>[20x]MSEKRVQPLARDAMAYVLAGGRG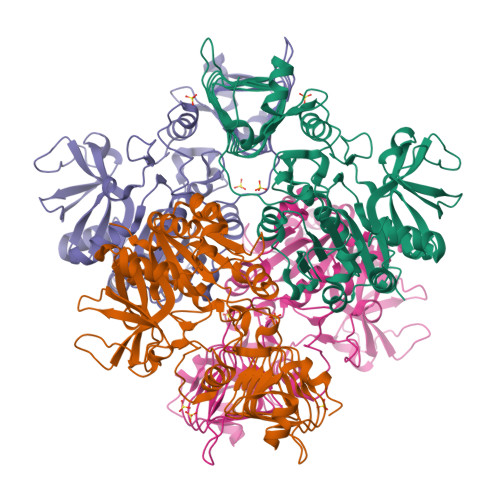SRLKELTDRRAKPAVYFGGKARIIDFALSNALNSGIRRIGVATQYKAHSLIRHLQRGWDFFRPERNESFDILPASQRVSETQWYEGTADAVYQNIDIIEPYAPEYMVILAGDHIYKMDYEYMLQQHVDSGADVTIGCLEVPRMEATGFGVMHVNEKDEIIDFIEKPADPPGIPGNEGFALASMGIYVFHTKFLMEALRRDAADPTSSRDFGKDIIPYIVEHGKAVAHRFADSCVRSDFEHEPYWRDVGTIDAYWQANIDLTDVVPDLDIYDKSWPIWTYAEITPPAKFVHDDEDRRGSAVSSVVSGDCIISGAALNRSLLFTGVRANSYSRLENAVVLPSVKIGRHAQLSNVVIDHGVVIPEGLIVGEDPELDAKRFRRTESGICLITQSMIDKLDL>[2x]SPKREYEERNVGKRLRLSEALKACSNILKDISSQRYRDLNHFFLKPVDVVALGLHDYYDVVKKAMDLSTIKTKLES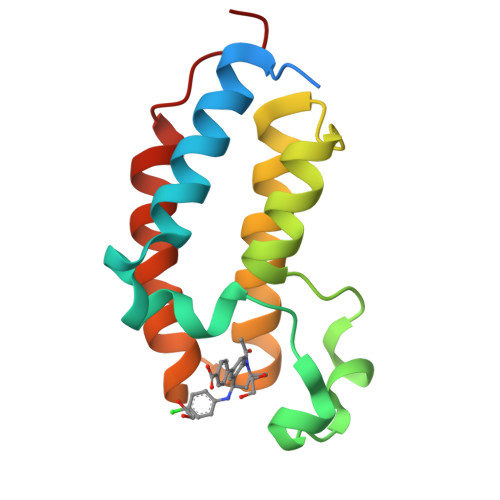GQYHTKYDFADDVRLMFNNCYKYNGEDSEVARVGKQLQAIFDENFAKVPDDES Dihydrofolate reductase (DHFR) is a critical enzyme in the recycling of folate cofactors that are essential for the synthesis of deoxythymidine monophosphate and several amino acids. Since inhibition of DHFR depletes the pool of available thymidine, it has proven to be an excellent drug target for rapidly proliferating bacteria, protozoa and cancer cells. Using high resolution structural information, we have developed a new class of antifolates characterized by a unique propargylic linker that shows activity against an expanded set of enzymes from important pathogens. Using a structure-based approach, a series of propargyl-linked antifolates were designed, synthesized and shown to possess highly potent antibacterial activity against both MRSA and S. pyogenes.

A series of biphenyl derivatives, 7–11, probe the deletion of both propargylic and C-ring methyl groups, extension of the C6 alkyl group and the role of the B-ring alkoxy substituent. As predicted from the previous structural analysis, removal of the hydrophobic branching substituents both at the propargyl position and the distal aryl ring is well tolerated. However, the contribution of the B-ring substituent was more pronounced (compare compounds 7 and 9), with a 2′-methoxy proving to be a more optimal placement, leading to a highly potent (2.4 nM and 5.9 nM) dual inhibitor of both S. aureus and S. pyogenes DHFR. In order to understand the divergence between activity in the biphenyl and heterocyclic series, crystal structures of S. aureus DHFR bound to compounds 7 or 25 were determined. Comparison of the structures of S. aureus DHFR:NADPH:7 and S. aureus DHFR:NADPH:1 shows minimal changes in the orientation of the three aryl rings present in both inhibitors. However, a major difference that accounts for the 18-fold improvement in potency for compound 7 against S. aureus DHFR is the presence of a hydrogen bond (3.5 Å) between the 2′-methoxy substituent in compound 7 and the hydroxyl group of Ser 49, an interaction that is precluded with the 3′-methoxy in compound 1.

>TLSILVAHDLQRVIGFENQLPWHLPNDLKHVKKLSTGHTLVMGRKTFESIGKPLPNRRNVVLTSDTSFNVEGVDVIHSIEDIYQLPGHVFIFGGQTLFEEMIDKVDDMYITVIEGKFRGDTFFPPYTFEDWEVASSVEGKLDEKNTIPHTFLHLIRKLEHHHHHHHH[2x]> PPPAIGQFWHVTDLHLDPTYHITDDHTKVCASSKGANASNPGPFGDVLCDSPYQLILSAFDFIKNSGQEASFMIWTGDSPPHVPVPELSTDTVINVITNMTTTIQSLFPNLQVFPALGNHDYWPQDQLPVVTS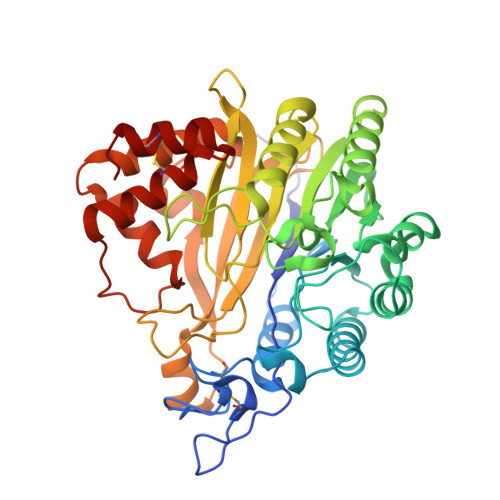KVYNAVANLWKPWLDEEAISTLRKGGFYSQKVTTNPNLRIISLNTNLYYGPNIMTLNKTDPANQFEWLESTLNNSQQNKEKVYIIAHVPVGYLPSSQNITAMREYYNEKLIDIFQKYSDVIAGQFYGHTHRDSIMVLSDKKGSPVNSLFVAPAVTPVKSVLEKQTNNPGIRLFQYDPRDYKLLDMLQYYLNLTEANLKGESIWKLEYILTQTYDIEDLQPESLYGLAKQFTILDSKQFIKYYNYFFVSYDSSVTCDKTCKAFQICAIMNLDNISYADCLKQLYIK> MSYKNATKPTETIMHANDAIQKTTASTRKPRLVVMVVGETARADHASFNGYQRATFPHMDKLIGLGQVHNFGNVTSCGTSTAYSVPCMFSYLGAEKYDVDTADYHENVIDTLDRLGVAILWRDNNSDSKGVMNRLPAKQYQDYKNSPLQG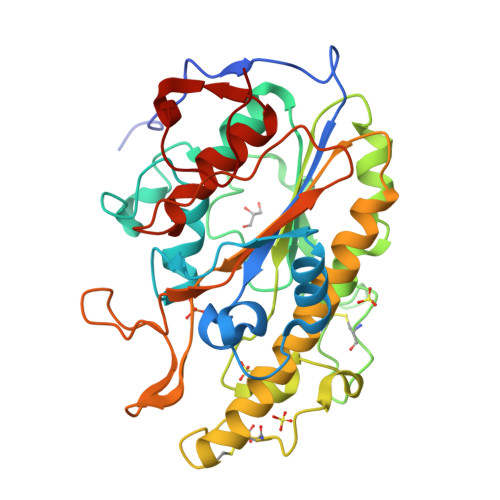GNNTICHTNPYDECRDVGMLVDLDDHVKAHANQDILIVLHQMGNHGPAYYKRYDDEFAQFLPVCTSSELAECERQTVINAYDNALLATDDFLKQTIDWLAAQTHADTAMLYLSDHGESLGEKGVYLHGMPKAFAPKEQLSIPALLWLGADTPFAVANSPTAGFSHDAITPTLLNLFDVSTQATADKTAFVNPLD>[4x]MLQIPQNYIHTRSTPFWNKQTAPAGIFERHLDKGTRPGVYPRLSVMHGAVKYLGYADEHSAEPDQ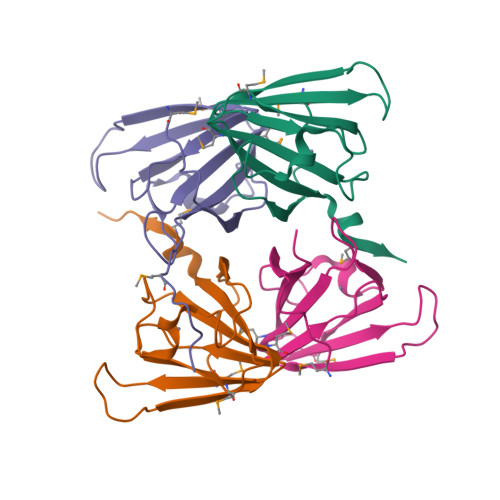VILIEAGQFAVFPPEKWHNIEAMTDDTYFNIDFFVAPEVLMEGAQQRKVIHNGKLEHHHHHH>[7x]XGEIAQALKEIAKALKEIAWALKEIAQAYKGX

αHBs are oligomers of 5 or more α-helical peptides that assemble into coiled-coil structures with central solvent-accessible channels. We targeted two properties of αHBs: oligomeric state, which directly affects the internal diameter of the channel; and the identities of channel-facing residues, which fine tune this dimension and introduce different chemistries. The αHBs are loaded with an environment sensitive dye (in this case, 1,6-diphenyl-1,3,5-hexatriene, DPH) that binds within the channels and fluoresces. Accordingly, challenging the array with analytes leads to differential displacement of the dye across the array to give a fluorescent fingerprint.

Despite the requirements for aliphatic residues at a and d, up to 40% of these can be changed to other side chains without compromising barrel integrity. We introduced mutations at one or two of these sites to generate four groups of αHB: Group I had entirely hydrophobic interiors, but with different sizes and shapes of channel; Groups II and III had polar uncharged or polar charged residues, respectively, at specific points along the channel; and Group IV had aromatic residues installed in their channels. Finally, seven Group IV designs incorporated single Tyr at a or d sites, or Trp residues at a sites. Finally, one third of the designs were crystallized and yielded 12 X-ray crystal structures, all of which were open αHBs with fully accessible channels. Conversely, the FAs generate signal through interactions with the more-hydrophobic and aromatic-containing channels (Group I and IV).> GLGQMLESMIDNTVRETVGAATSRDALPNTEASGPTHSKEIPALTAVETGATNPLVPSDTVQTRHVVQHRSRSESSIESFFARGACVTIMTVDNPASTTNKDKLFAVWKITYKDTVQLRRKLEFFTYSRFDMELTFVVTANFTETNNGHALNQVYQIMYVPPGAPVPEKWDDYTWQTSSNPSIFYTYGTAPARISVPYVGISNAYSHFYDGFSKVPLKDQSAALGDSLYGAASLNDFGILAVRVVNDHNPTKVTSKIRVYLKPKHIRVWCPRPPRAVAYYGPGVDYKDGTLTPLSTKDLTTY;> SPNIEACGYSDRVLQLTLGNSTITTQEAANSVVAYGRWPEYLRDSEANPVDQPTEPDVAACRFYTLDTVSWTKESRGWWWKLPDALRDMGLFGQNMYYHYLGRSGYTVHVQCNASKFHQGALGVFAVPEMCLAGDSNTTTMHTSYQNANPGEKGGTFTGTFTPDNNQTSPARRFCPVDYLLGNGTLLGNAFVFPHQIINLRTNNCATLVLPYVNSLSIDSMVKHNNWGIAILPLAPLNFASESSPEIPITLTIAPMCCEFNGLRNITLPRLQ;> GLPVMNTPGSNQYLTADNFQSPCALPEFDVTPPIDIPGEVKNMMELAEIDTMIPFDLSATKKNTMEMYRVRLSDKPHTDDPILCLSLSPASDPRLSHTMLGEILNYYTHWAGSLKFTFLFCGSMMATGKLLVSYAPPGADPPKKRKEAMLGTHVIWDIGLQSSCTMVVPWISNTTYRQTIDDSFTEGGYISVFYQTRIVVPLSTPREMDILGFVSACNDFSVRLLRDTTHIEQKALAQ;> XGAQVSSQKVGAHENSNRAYGGSTINYTTINYYRDSASNAASKQDFSQDPSKFTEPIKDVLIKTAPMLN;> DVVVQAPTQVPGFLGDSVTLPCYLQVPNMEVTHVSQLTWARHGESGSM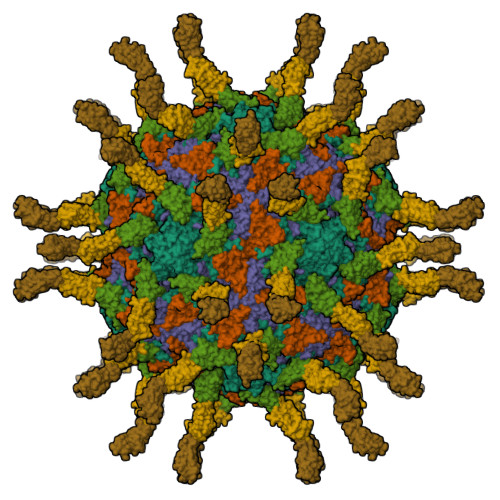AVFHQTQGPSYSESKRLEFVAARLGAELRNASLRMFGLRVEDEGNYTCLFVTFPQGSRSVDIWLRVLA;> LAKPQNTAEVQKVQLTGEPVPMARCVSTGGRPPAQITWHSDLGGMPNTSQVPGFLSGTVTVTSLWILVPSSQVDGKNVTCKVEHESFEKPQLLTVNLTVYYP;> YPPEVSISGYDNNWYLGQNEATLTCDARSNPEPTGYNWSTTMGPLPPFAVAQGAQLLIRPVDKPINTTLICNVTNALGARQAELTVQVKEGP1-chloropentane 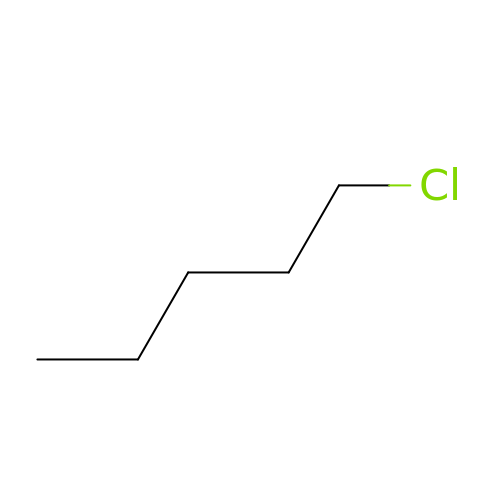| C5 H11 Cl | SQCZQTSHSZLZIQ-UHFFFAOYSA-N>[2x]GSHMSDSNTITSFQVDCYLWHIRKLLSMRDMCDAPFDDRLRADQAALKGRGSTLGLDLRVATMEGKKIVEDILKSET

Encoded by the smallest of the eight viral genome segments, NS1 is a multifunctional RNA-binding protein, which is considered the main weapon of the virus to antagonize the innate immune response of the host and to ensure viral replication in a hostile anti-viral environment. While the effector domain is to some extent dispensable for the biological activities of NS1, the RBD plays an essential role in several activities that require the interaction of NS1 with viral and non-viral RNAs. This is best illustrated by the total loss of pathogenicity conferred by the alanine substitution of Arg38 and Lys41, the two main residues involved in binding of RNAs by NS1.

As expected, the double substitution R38A/K41A, either in the H7N1 or H5N1-origin RBD, abolished their binding to both RNAs. Surprisingly, the negative impacts of the double substitution (R38A-K41A) were very different for the H5N1 and H7N1 RBDs. Under the stringent binding conditions that we used, the mutant H7N1-RBD was unable to form a stable complex with AWFC01. In order to search for complementary clues for the apparent sequence specificity of the H7N1 RBD for AWFC01, we solved the 3D structures of two other complexes: (i) R38A-K41A double mutant H7N1 RDB with AWFC01 (aaH7N1-RBD/AWFC01) and (ii) wild type H7N1 RBD, with the slightly modified nonspecific RNA “ZKO*” (wtH7N1-RBD/ZKO*). While the two complexes crystallized in different conditions and space groups, noteworthy similarities were observed with low rmsd values of 0.33 Å for the proteins and 0.71 Å for the RNA. When comparing by superimposition the structures of the three RBD-RNA complexes, subtle structural differences were identified, mainly for the RNA molecule. Relative to the wtH7N1-RBD/AWFC01 complex, the RNAs in complexes aaH7N1-RBD/AWFC01 and wtH7N1-RBD/ZKO* differ by rmsd values of 2.00 Å and 2.21 Å, respectively, whereas the difference is much smaller as regards the RBD (rmsd of 0.26 Å and 0.33 Å, respectively). Surprisingly, this revealed that in the high affinity dsRNA (AWFC01), the RNA axis is bent in a non-symmetrical fashion, whereas in the two other complexes (aaH7N1-RBD/AWFC01 and wtH7N1-RBD/ZKO*), the RNA axis bend is distributed symmetrically from the centre of the duplex.>SGDLYRACLYERVLLALHDRAPQLKISDDRLTVVGEKGYSMVRASHGVRKGAWYF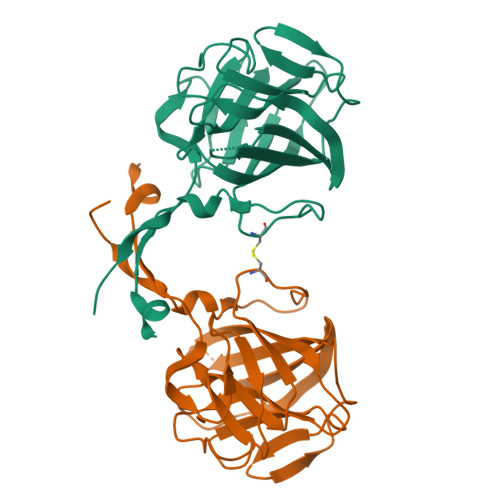EITVDEMPPDTAARLGWSQPLGNLQAPLGYDKFSYSWRSKKGTKFHQSIGKHYSSGYGQGDVLGFYINLPEDTISGRGSSEIIFYKNGVNQGVAYKDIFEGVYFPAISLYKSCTVSINFGPCFKYPPKDLTYRPMSDMGWGAVVEHTLADVLYHVETE[2x]While most SAM riboswitches strongly discriminate between SAM and SAH, the SAM/SAH riboswitch responds to both ligands with similar apparent affinities. The riboswitch forms an H-type pseudoknot structure with coaxial alignment of the stem–loop helix (P1) and the pseudoknot helix (PK). An additional three base pairs form at the non-open end of P1, and the ligand is bound at the interface between the P1 extension and the PK helix. Binding SAM or SAH stabilizes the PK helix, so structuring the Shine–Dalgarno sequence, sequestering it and preventing initiation of translation (OFF state).

The structures were unaffected by crystal contacts: the structure of the riboswitch bound to SAM was solved in space groups P312 and C2, with an all-atom RMSD of 0.26 Å. Electron density for the remaining part of the methionine is not visible for the bound SAM ligand, but is observable for the bound dCSAH showing that the primary amine is hydrogen bonded to U23 O4 just as it is for SAH. The sulfur atom is 3.8 Å away from the nearest RNA atom, leaving enough space to accommodate the SAM methyl group without steric clash, and the open binding site will readily accommodate the trajectory of the chain with a planar thioether (SAH) or tetrahedral sulfonium (SAM). In addition there is no electrostatic interaction with the positively charged sulfonium ion as there is in the SAM-II and V riboswitches. The structure therefore explains why this riboswitch binds both SAM and SAH with similar affinities.

>[2x]GGUCACAACGGCUUCCUGGCGUGACC;>AUUGGAGCA[2x]>[6x]MSQLTHINAAGEAHMVDVSAKAETVREARAEAF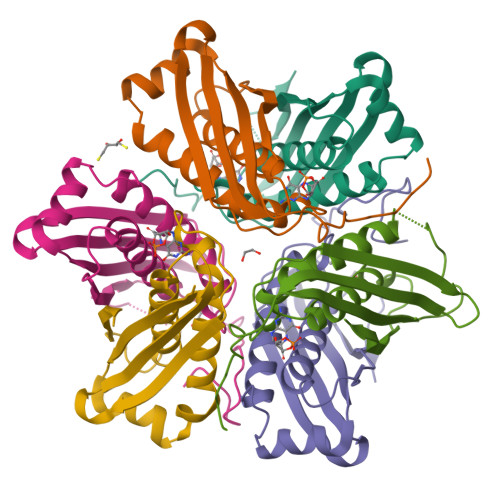VTMRSETLAMIIDGRHHKGDVFATARIAGIQAAKRTWDLIPLCHPLMLSKVEVNLQAEPEHNRVRIETLCRLTGKTGVEMEALTAASVAALTIYDMCKAVQKDMVIGPVRLLAKSGGKSGDFKVEADD> GPGSKKRQWALEDFEIGRPLGK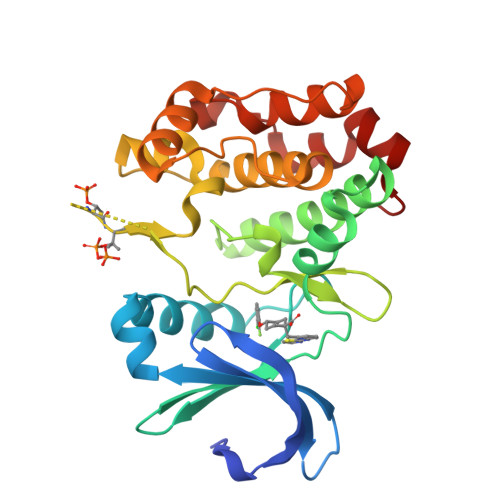GKFGNVYLAREKQSKFILALKVLFKAQLEKAGVEHQLRREVEIQSHLRHPNILRLYGYFHDATRVYLILEYAPLGTVYRELQKLSKFDEQRTATYITELANALSYCHSKRVIHRDIKPENLLLGSAGELKIADFGWSVHAPSSRRTTLCGTLDYLPPEMIEGRMHDEKVDLWSLGVLCYEFLVGKPPFEANTYQETYKRISRVEFTFPDFVTEGARDLISRLLKHNPSQRPMLREVLEHPWITANSSKP>[2x]GSGSPLAQQIKNTLTFIGQANAAGRMDEVRTLQENLHPLW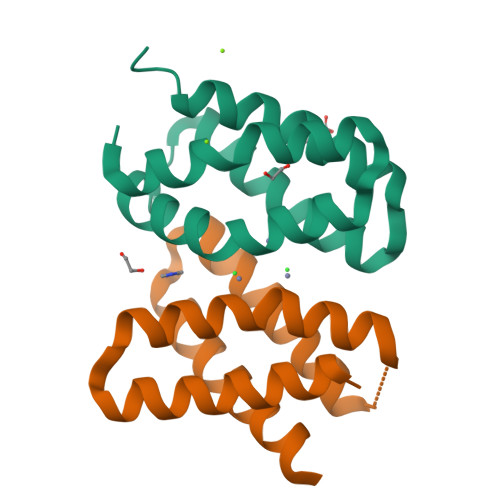HEYFQQTEGSGGSPLAQQIEYGHVLIHQARAAGRMDEVRRLSENTLQLMKEYFQQSD>[2x]GSMDLYRQSLEIISRYLREQATGAKDTKPMGRSGATSRKALETLRRVGDGVQRNHETAFQGMLRKLDIKNEDDVKSLSRVMIHVFSDGVTNWGRIVTLISFGAFV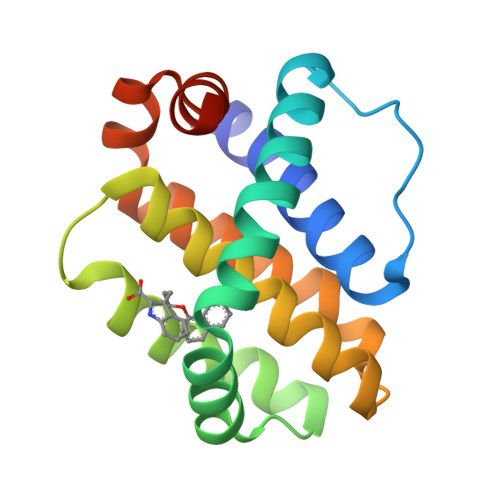AKHLKTINQESCIEPLAESITDVLVRTKRDWLVKQRGWDGFVEFFHVEDLEG The TipA (thiostrepton-induced protein A) class of transcriptional regulators found in diverse bacteria is viewed as a minimal autoregulated MDR system. TipA proteins belong to a subset of the superfamily of mercuric ion resistance (MerR)–like transcriptional regulators that contain an N-terminal helix-turn-helix (HTH) motif followed by an intermediate linking coiled-coil (PF00376 MerR and PF13411 MerR_1 families in the Pfam database) and a C-terminal TipAS-type effector domain (PF07739 TipAS family in the Pfam database). In addition to S. lividans, TipA-class proteins have also been reported to have crucial regulatory functions in other species such as Mta (multidrug transporter activation protein) from Bacillus subtilis, stationary-phase regulation of KatG protein (SkgA) from Caulobacter crescentus, and AlbA (albicidin resistance protein) containing two tandem TipAS domains from Klebsiella oxytoca. Structural and biochemical analyses indicated that the interaction of TipA regulators with promoter DNA is hindered in the apo state and revealed an unexpected activation mechanism in which drug binding induces conformational turnover of the TipAS domain to release the N-terminal HTH motif for promoter DNA binding and subsequent transcriptional activation, during which the α6–α7 region may serve as a key switch element to drive the global transition.

As a result, diffraction-quality crystals of SkgA were obtained, and the structure was determined at a resolution of 2.5 Å using the single-wavelength anomalous dispersion phasing method. Although full-length SkgA (residues 1–255) protein was used for crystallization, only residues 1–138 were observed in the final structure. The established structure consists of the N-terminal MerR-type HTH motif, coiled-coil region, and the initial two α-helices of the C-terminal TipAS domain, whereas the rest of the TipAS domain was still invisible in the current model, probably because of structural flexibility or diffraction damage. Because MerR family proteins reportedly function as dimers and SkgA protein also exhibits a dimer conformation in solution, a dimeric SkgA structure was established by combining two molecules from two adjacent asymmetric units for subsequent analysis. Remarkably, apart from the coiled-coil α5 helices, the α6–α7 region and N-terminal domain are also involved in the dimeric interface. Fifteen residues of the α6–α7 region of each protomer interact with the N-terminal domain of the other protomer via hydrogen bonding, ionic bonding, and hydrophobic interactions, which contribute to stabilization of the conformation of the α6–α7 region. Eleven residues of the N-terminal α1–α2 region exhibit interactions with ten residues of the α6–α7 region via hydrophobic interactions and three hydrogen bonds formed by residue pairs Tyr4–Asp117, Ser16–Glu133, and Tyr23–His132.

> MHHHHHHMSVYTVKQMARLSGVSVRALHHYDAIGLLKPRAVGANGYRYYDRQDLLRLQQILFHRALETPLKDIQAALDQPGFDLAAALRAQRERLAAQAERYARLVDVVDRTLADLEGDETMDDKHLFEGFDPEKQARHEAWLVEHYGDEATRRIADAKAGMKSWGKKDWSQFQEEAKAIEHDLAKALTQGLPVDSAPVTAIMRRHWAWVGRSWNREPTPDAFAGLGHLYQANPEFTARYEAIAPGLTEYFSEAMRAFARGR> GPPDLGTDDDDKAMADIASCTTQEKTAPVISVAEQAVPSISEIDRSYLLSSDRLTEVDGNTLDVASEEQVAALKAQFENLKDGDEVVIPNGKYANLGQVTITANDVTIRAEQAGAAWLTGLIQFELKGDDITLDGLVFTEGGPNERFGAVRMMGNGNTLQNSTFYYFNHDYTYEPDERRSEYPKYLWVSLWGKDGKVINNRFEGKQKRGTLIGVQKDDTP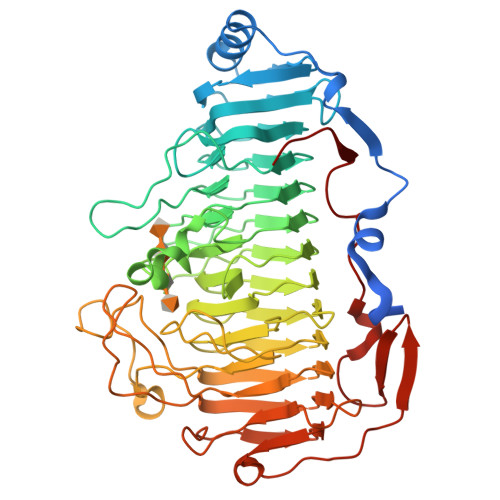DNHLIANNIFMDQKPNQFNEFDIKEAIRYNGNSWEAIRIGDSKSSQWDSSSKFVNNLMIDMDGERELISIKSGDNTISGNTIFQSAALISLRHGKGNTVENNMILGNEKRLTGGIRIYDEDHVIRNNYIANTRGRDGVIEGNADLRGGIVINTGIIDVANGEQLDQSVKGKELNKQWTPKNITIENNSLVDTEWGIVYGNQSHRVSLFNNAEVEGIYAGVDIAFKHNVVDNSQTPEFVSVRATHDFPLVGATYTDETYVGQVTDSELIESYSVELPKVTVENGLNAYQGEGADVSKLSVVTAETAGPDYVLENTTK>MNTLPSQVWRTNIGSAPSQLLNYIDGNFVTSASSFANINPVNGKLISDVFEADAKQVNEAVVAAQNALKGPWGKLSVQDRAALIHKIADGIQARFEEFVAAEVADTGRPVHQARTLDIPRAIANFRTFADLAKTSHTDLFEMSTSDGSGALNYTVRKPLGVIGVISPWNLPLLLFTWKVAPALACGNTVVAKPSEESPSSATLLAEVMHDAGVPPGVFNLIHGFGKDSAGEFLTQHPGISALTFTGESKTGSTIMKAVADGVKEVSFELGGKNAAVVFADADLDAAIEGVLRSSFTNSGQVCLCSERVYVHRSIFDEFVSGLKVEAERLVVGYPDQDGVNMGPLISHGHRDKVLSYYRLAVDEGATVVTGGGVPKFNDERDQGAYVQPTIWTGLSDKARCVTEEIFGPVCHISPFDDEDEVINRVNDSNYGLACAIWTTNLSRAHRVSRQIHVGLVWVNTWYLRDLRTPFGGVKLSGLGREGGRFSMDFYSDIANICIKI[4x]

One enzyme in particular, 2-aminomuconate-6-semialdehyde dehydrogenase (AMSDH), is responsible for oxidizing the unstable metabolic intermediate 2-aminomuconate-6-semialdehyde (2-AMS) to 2-aminomuconate (2-AM). On the basis of sequence alignment, AMSDH is a member of the hydroxymuconic-semialdehyde dehydrogenase (HMSDH) family under the aldehyde dehydrogenase (ALDH) superfamily. The complete AMSDH model includes four polypeptides per asymmetric unit describing one homotetramer. Each monomer of AMSDH contains three domains: a subunit interaction domain, a catalytic domain and an NAD+ binding domain.

Structures of AMSDH in ternary complex with co-substrate NAD+ and its primary substrates were obtained by soaking co-crystallized AMSDH-NAD+ crystals with 2-AMS and 2-HMS, respectively. Extra density that fits with the corresponding substrate molecule was observed in the active site of each subunit. Binding of the primary substrates introduced minimal change to the protein structure; the r.m.s.d. for the superimposed structures of substrate-free with 2-AMS- and 2-HMS-bound ternary complex structures are 0.170 and 0.276 Å, respectively. These two primary substrates bind to AMSDH in an identical fashion, with two arginine residues, Arg120 and Arg464, playing an important role in stabilizing the substrate by forming two sets of bifurcated hydrogen bonds with one of the carboxyl oxygens and the 2-amino or hydroxyl group of 2-AMS or 2-HMS, respectively. The observation of two hydrogen bonds being donated by the active site arginines to the 2-amino group of 2-AMS indicates that in the substrate-bound form, 2-AMS may be in its 2-imine rather than 2-enamine tautomer, as an amino group unlikely to accept two hydrogen bonds. 2-AMS is an unstable compound which decays with a t1/2 of about 9 s at pH 7.5 and 37 °C or 35 s at pH 7.0 and 20 °C. Notably, this is its first reported structure. It appears to be stabilized in the enzyme active site in its imine tautomer by forming two sets of bifurcated hydrogen bonds with Arg120 and Arg464 so that the electrocyclization reaction cannot occur. In the ternary complex structures, Cys302 is located at an ideal position to initiate catalysis, which is the attacking state. In the two ternary complex structures, the distance between the sulfur of Cys302 and the C6 of the substrate is ~3.3 Å. Interestingly, in both substrate-bound structures, Glu268 becomes more flexible and exhibits much weaker electron density and increased side chain B-factors compared with average protein B-factors: 37.8 Å2/28.5 Å2 and 66.37 Å2/39.7 Å2.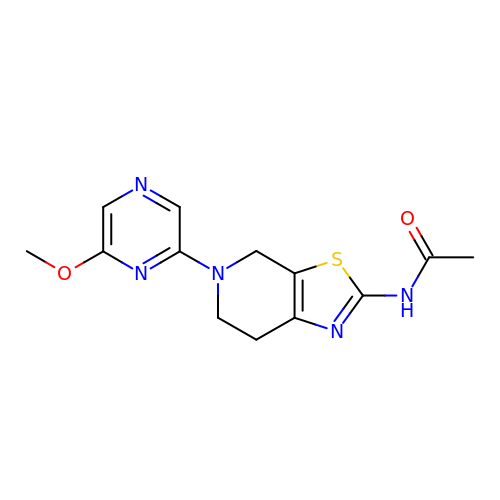N-[5-(6-methoxypyrazin-2-yl)-4,5,6,7-tetrahydro[1,3]thiazolo[5,4-c]pyridin-2-yl]acetamide | C13 H15 N5 O2 S | YGHXBCAMJWBJDS-UHFFFAOYSA-N> MSLEEQRTRDELKHKLLDLNQLHEQLAELRTICPSLLKLLHPETGTSRKFEKSAQEAIEKVNSFYTHLKSSQNVFDYAEKSLQADSSNLLPTYLYNSEDLSNDTENNETKSINGKSALDLKEPHHSELHDNDNFQNSDINIES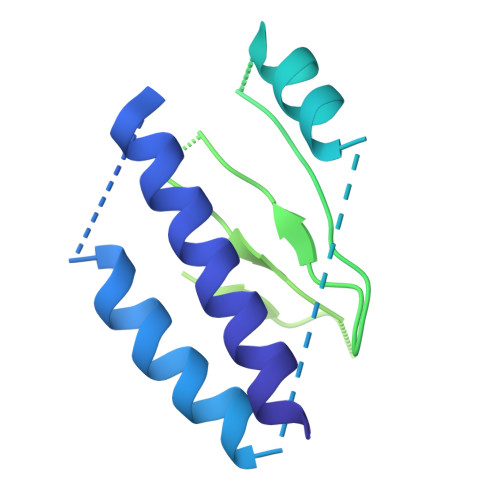FKGDIEASGSILTTHENKSFTLKLANELEFIFFHDTRGKFSVYCSSSKDDAITFSINRNNNFLGNLWSLMPKILDYQHLYSKPCDFCKSLISPVYLELPSVRRNANSTVKPTSKDILALHAECVPAQSDL ethyl ({4-oxo-3-[3-(pyrrolidin-1-yl)propyl]-3,4-dihydro[1]benzothieno[3,2-d]pyrimidin-2-yl}sulfanyl)acetate | C21 H25 N3 O3 S2 | 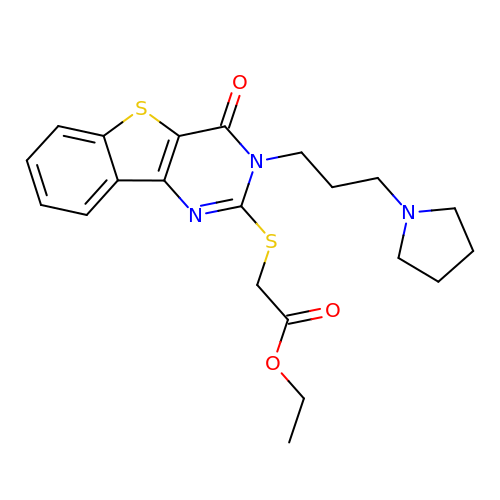SKDRHRAYBYQVNU-UHFFFAOYSA-N>[2x]GAAGSPEEDMEDRVRIDPVAGGYYPSISPSAQTRGATPDGETLKDRPIFLLEDGSTIRLVVYDDAKNLLEEYSKAYLVRNAGTSGSSL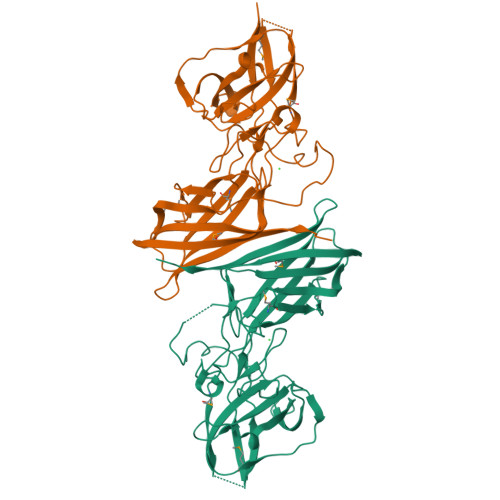LYPCEVDDNGAVISSSSTPLYMKAGTYYFRILSPAKALNSKGFVNIGNGEYLLATDDRYTQTAMTAVTITKIDEGGTLNNVQTLYLPPIINQTARMQFTVRAGEGVHTLEMLAEGIEISGIQQPLDNTTSFDWVNGDVLPVKVGDQSASVRITQATRNADNSLVAHTGVLPTDARSHSISVLLNLKVNGNPTQYQMLLTGLYLTAGHSYNYTATVKISNGVTVLTWQNRSWTENVVMDK>GEEQMRLPSADVYRFAEPDSEENIIFEENMQPKAGIPIIKAGTVIKLIERLTYHMYADPNFVRTFLTTYRSFCKPQELLSLIIERFEIPEPEPTEADRIAIENGDQPLSAELKRFRKEYIQPVQLRVLNVCRHWVEHHFYDFERDAYLLQRMEEFIGTVRGKAMKKWVESITKIIQRKKIARDNGPGHNITFQSSPPTVEWHISRPGHIETFDLLTLHPIEIARQLTLLESDLYRAVQPSELVGSVWTKEDKEINSPNLLKMIRHTTNLTLWFEKCIVETENLEERVAVVSRIIEILQVFQELNNFNGVLEVVSAMNSSPVYRLDHTFEQIPSRQKKILEEAHELSEDHYKKYLAKLRSINPPCVPFFGIYLTNIL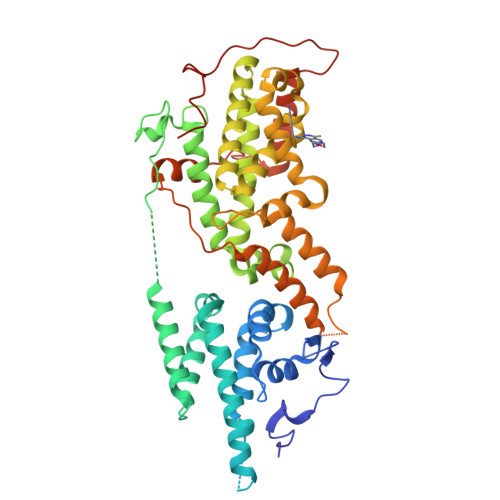KTEEGNPEVLKRHGKELINFSKRRKVAEITGEIQQYQNQPYCLRVESDIKRFFENLNPMGNSMEKEFTDYLFNKSLEIEPRNPKPLPRFPKKYSYPLKSPGVRPSNPRPGT[2x]> MRGSFVEMVDNLRGKSGQGYYVEMTVGSPPQTLNILVDTGSSNFAVGAAPHPFLHRYYQRQLSSTYRDLRKGVYVPYTQGKWEGELGTDLVSIPHGPNVTVRANIAAITESDKFFINGSNWEGILGLAYAEIARPDDSLEPFFDSLVKQTHVPNLFSLQLCGAGFPLNQSEVLASVGGSMIIGGIDHSLYTGSLWYTPIRREWYYEVIIVRVEINGQDLKMDCKEYNYDKSIVDSGTTNLRLPKKVFEAAVKSIKAASSTEKFPDGFWLGEQLVCWQAGTTPWNIFPVISLYLMGEVTNQSFRITILPQQYLRPVEDVATSQDDCYKFAISQSSTGTVMGAVIMEGFYVVFDRARKRIGFAVSACHVHDEFRTAAVEGPFVTLDM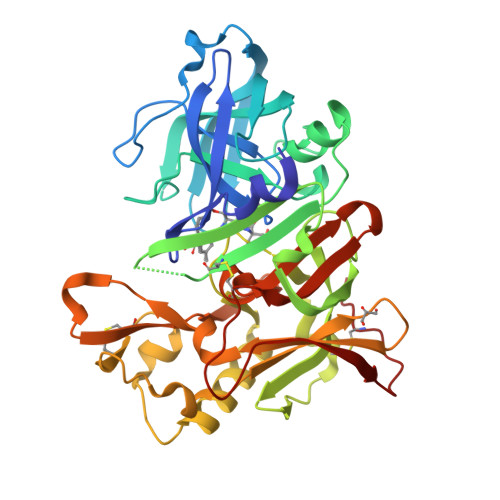EDCGYN> MSKPGRTILASKVAETFNTEIINNVEEYKKTHNGQGPLLVGFLANNDPAAKMYATWTQKTSESMGFRYDLRVIEDKDFLEEAIIQANGDDSVNGIMVYFPVFGNAQDQYLQQVVCKEKDVEGLNHVYYQNLYHNVRYLDKENRLKSILPCTPLAIVKILEFLKIYNNLLPEGNRLYGKKCIVINRSEIVGRPLAALLANDGATVYSVDVNNIQKFTRGESLKLNKHHVEDLGEYSEDLLKKCSLDSDVVITGVPSENYKFPTEYIKEGAVCINFACTKNFSDDVK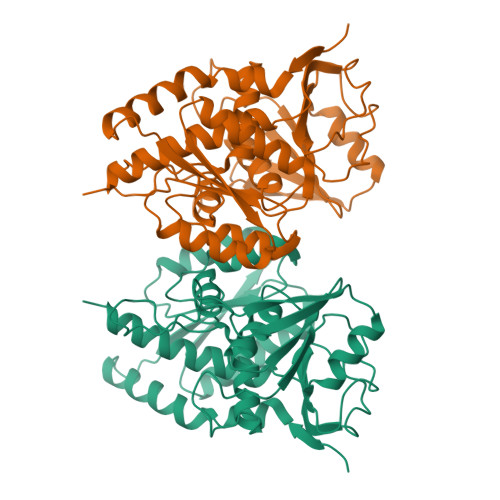EKASLYVPMTGKVTIAMLLRNMLRLVRNVELSKEK CRISPR-RNA (clustered, regularly, interspaced, short palindromic repeats-RNA) along with Cas proteins assemble into RNA-guided adaptive immune complexes in prokaryotes. These CRISPR–Cas systems defend bacteria and archaea against the invasion of foreign genetic elements. The type I-C subtype is one of the most prevalent systems found in bacteria. Interestingly, type I-C Cascade only contains three unique Cas proteins in its operon: Cas5c, Cas7, and Cas8c3.

To understand the molecular basis for small-subunit incorporation, we determined a 3.1 Å resolution cryo-EM reconstruction of the type I-C Cascade complex, suitable for de novo model building (except for the flexible N terminus of Cas8c). The overall architecture of the complex resembles a caterpillar. Seven Cas7 subunits form a right-handed helical filament around the crRNA and Cas5c sits at the base of the complex. Cas5c and Cas7.7 clamp around the crRNA 5′-handle (nucleotides U1–G12), forcing it into a hooked conformation (inset). Cas5c residues “pinch” the phosphate groups within the crRNA backbone on either side of the U5 nucleobase, inducing a sharp (33°) kink. Nucleotides on either side of this kink are captured by a network of Cas5c π–π stacking interactions, while Cas7.7 makes non-specific contacts with the phosphate backbone. These highly conserved interactions (inset) suggest that the 5′ end of the crRNA handle is critical for type I-C Cascade assembly. Despite these differences, type I-C Cas7 maintains a highly conserved region of positive residues to form non-specific interactions with the phosphate backbone of the crRNA. The belly of the complex contains the large subunit, Cas8c, and two copies of the SSU, which nucleate and are derived from the C-terminal domain of Cas8c (residues 489–612). Remarkably, the electrostatic surface potential of the type I-C Cascade reveals a contiguous channel of positively charged residues that runs along the length of this minor filament from the large subunit.

> TYGIRLRVWGDYACFTRPEMKVERVSYDVMPPSAARGILEAIHWKPAIRWIVDRIHVLRPIVFDNVRRNEVSSKIPKPNPATAMRDRKPLYFLVDDGSNRQQRAATLLRNVDYVIEAHFELTDKAGAEDNAGKHLDIFRRRARAGQSFQQPCLGCREFPASFELLEGDVPLSCYAGEKRDLGYMLLDIDFERDMTPLFFKAVMEDGVITPPSRTSPEVRA;>[7x]MTAIANRYEFVLLFDVENGNPNGDPDAGNMPRIDPETGHGLVTDVCLKRKIRNHVALTKEGAERFNIYIQEKAILNETHERAYTACDLKPEPKKLPKKVEDAKRVTDWMCTNFYDIRTFGAVMTTEVNCGQVRGPVQMAFARSVEPVVPQEVSITRMAVTTKAEAEKQQGDNRTMGRKHIVPYGLYVAHGFISAPLAEKTGFSDEDLTLFWDALVNMFEHDRSAARGLMSSRKLIVFKHQNRLGNAPAHKLFDLVKVSRAEGSSGPARSFADYAVTVGQAPEGVEVKEML;> WENTSYILGVDAKGKQERTDKCHAAFIAHIKAYCDTADQDLAAVLQFLEHGEKDLSAFPVSEEVIGSNIVFRIEGEPGFVHERPAARQAWANCLNRREQGLCGQCLITGERQKPIAQLHPSIKGGRDGVRGAQAVASIVSFNNTAFESYGKEQSINAPVSQEAAFSYVTALNYLLNPSNRQKVTIADATVVFWAERSSPAEDIFAGMFDPPSTTAKPESSNGTPPEDSEEGSQPDTARDDPHAAARMHDLLVAIRSGKRATDIMPDMDESVRFHVLGLSPNAARLSVRFWEVDTVGHMLDKVGRHYRELEIIPQFNNEQEFPSLSTLLRQTAVLNKTENISPVLAGGLFRAMLTGGPYPQSLLPAVLGRIRAEHARPEDKSRYRLEVVTYYRAALIKAYLIRNRKLEVPVSLDPARTDRPYLLGRLFAVLEKAQEDAVPGANATIKDRYLASASANPGQVFHMLLKNASNHTAKLRKDPERKGSAIHYEIMMQEIIDNISDFPVTMSSDEQGLFMIGYYHQRKALFTKKNKEN;>[2x]VSLDPARTDRPYLLGRLFAVLEKAQEDAVPGANATIKDRYLASASANPGQVFHMLLKNASNHTAKLRKDPERKGSAIHYEIMMQEIIDNISDFPVTMSSDEQGLFMIGYYHQRKALFTKKNKEN> MSQSNRELVVDFLSYKLSQKGYSWSQFSDVEENRTEAPEETEAERETPSAINGNPSWHLADSPAVNGATGHSSSLDAREVIPMAAV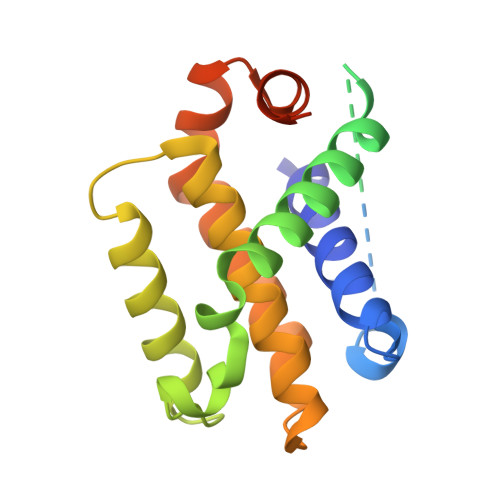KQALREAGDEFELRYRRAFSDLTSQLHITPGTAYQSFEQVVNELFRDGVNWGRIVAFFSFGGALCVESVDKEMQVLVSRIASWMATYLNDHLEPWIQENGGWDTFVDLYGNNAAAESRKGQERFN>HHHHHHKASKRTQLRNELIKQGPKRP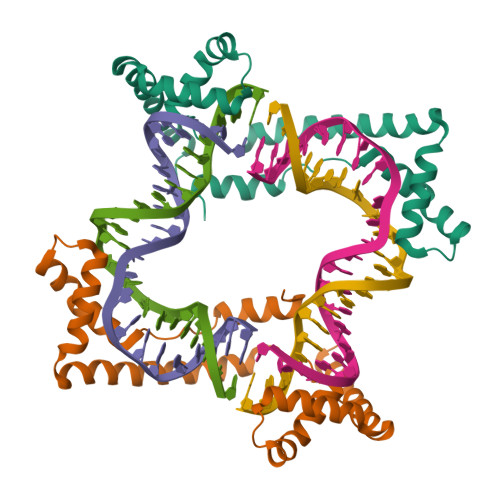TSAYFLYLQDHRSQFVKENPTLRPAEISKIAGEKWQNLEADIKEKYISERKKLYSEYQKAKKEFDEKLPPKKPAGPFIKYANEVRSQVFAQHPDKSQLDLMKIIGDKWQSLDQSIKDKYIQEYKKAIQEYNARYPLN[4x]> MAHHHHHHMQLSSLTAVSPVDGRYAGKTSSLRPIFSEYGLIRFRVMVEVRWLQRLAAHAGIPEVAPFSAEANALLDSLASDFQLEHAERIKEIERTTNHDVKAVEYLLKEQAAKLPELAAVSEFIHFACTSEDINNLSHALMLREGRDSVLLPLMRQIAEAIRELAVKLADVPMLSRTHGQPASPTTLGK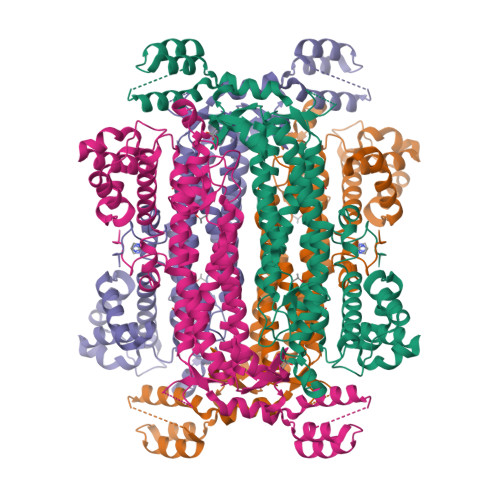ELANVVYRLERQIKQVAGIELLGKINGAVGNYNAHLSAYPEVDWEANARQFIEGDLGLTFNPYTTQIEPHDYIAELFDAIARFNTILIDFDRDVWGYISLGYFKQKTVAGEIGSSTMPHKVNPIDFENSEGNLGIANALFQHLASKLPISRWQRDLTDSTVLRNLGVGIAHSIIAYEASLKGIGKLELNAQRIAEDLDACWEVLAEPVQTVMRRYGVENPYEKLKELTRGKGISAEALQTFIEELAIPAEAKVELKKLTPAGYVGNAAAQAKRI>THPDISVDVLVIGAGPTGLGAAKRLNQIDGPSWMIVDSNETPGGLASTDVTPEGFLYDVGGHVIFSHYKYFDDCLDEALPKEDDWYTHQRISYVRCQGQWVPYPFQNNISMLPKEEQVKCIDGMIDAALEARVANTKPKTFDEWIVRMMGTGIADLFMRPYNFKVWAVPTTKMQCAWLGERVAAPNLKAVTTNVILGKTAGNWGPNATFRFPARGGTGGIWIAVANTLPKEKTRFGEKGKVTKVNANNKTVTLQDGTTIGYKKLVSTMAVDFLAEAMNDQELVGLTKQLFYSSTHVIGVGVRGSRPERIGDKCWLYFPEDNCPFYRATIFSNYSPYNQPEASKKLPTMQLADGSRPQSTEAKEGPYWSIMLEVSESSMKPVNQETILADCIQGLVNTEMLKPTDEIVSTYHRRF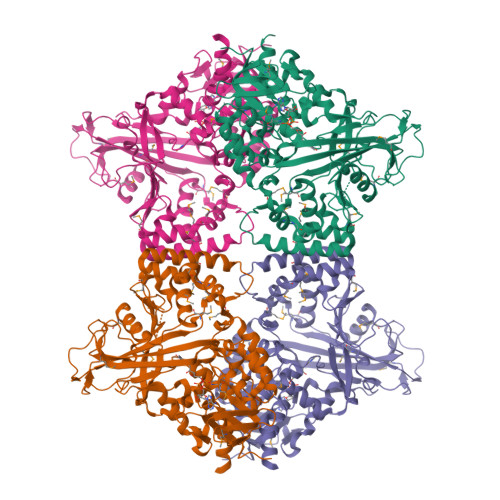DHGYPTPTLEREGALTQILPKLQDKDIWSRGRFGSWRYEVGNQDHSFMLGVEAVDNIVNGAVELTLNYPDFVNGRQNTERRLVDGAQVFAKSKAQ[4x]> MRRRIPSRTPGSGAKQKSWFPRRSL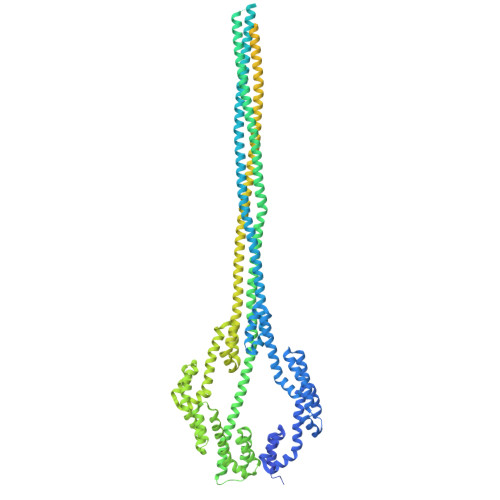QVLLSAGMLSGLLGTPAALAAEPAPLPANVRADIVGYWETGGAGLKAAAEQALLGGDEAIRKFLADAPSIQHDDNRIDAARMAMTGGSGLRQAAKDAIRLSPAELEKFLLYGYEEPLDDDHKVEIARLINLGGPGVREAGKAALQGTAEERELFLNSGQYTAQQDDNRVDVARLATTGGPNVQAAAKVALRGTPEDMVEFLEVGQFTARNRDQEHATIAELIKQAELAGKQADDARKTAEESSKKAVDASQLAKEAAQKAAEETEAAKDDSQKAAVKAKQAADAARAAADAAQEAIGSANAANRAARRAALAAAQTASAATAAAEAANKAYKAAIAAAGDEGKADEAKEAAKQARAAADAATKSGLAAENAGLASAAAATASTAAKSASSNARAAAGAAEEANQHADAAGVHSNEAALAAAEARRHADAADRAADRSSALAQRAATAAYGARDAANSAAEHANKAADYADESAAHAGDSAAYAATAKRNAQAAQEAAKTATAAVTKANEIFKLARETETANLETRTDAAIERARSMKSASETSITASATTQVEALALNDTATELAKEASRPDIDVQATAAKGRQLAMQAMKLLGPWHQEAAARALSGTDQDVLDYLRTRWKEANHNDIRQQIVDLSTQSPYASVRTAAAEALNGTPEQIEAFHTTGQYTAGSDDMKVDVARLANTGGPGVSQAAKTALADGTGKTLATFLQIGQYGERLSDEKVVTARLAETGSPEVQAAAKIALAGPPELLHEFVTTGQYMAKRKDDLADVHVNQVERLLAEGSLIAAEANEDAWRATEAAATAEGAAADAATAAEKAEASAAQAKQHAADADASADAATRSAADAAASAATARDAADRAAQDATAAENSAAEAAFSAAYARDSASKADDAADRARASALAAGKSADEAEAEAKEAWKTTRALAEKEAEEARRKAAEERKRQQEQAGEPKRVCIPHPTRETMIPIMPCAASPDDSMIMPGPVDPTIRAVVWELAGLNDIKACIDKPLSGNCVMAVVGVTPWGKFKLVSKLGNGLDAVKDARGARRTVACLTGAAHSFPAGTRVLMADGTRRSIEQIEAGDLVTATDPTTGETGARTVTRTIHTPDDRNFTDVALADGSTLTSTTHHPYWSQNDQTWKNAGDLEAGDTLRTPQNTAVVIAATHDWPGLQDAYDLTVDGFHSYYVSTGTTDVLVHNNDNPCPDWVSKAWKKLPKRKSGDPTSGYVFEADGTLVWDSVLTSGRSPLSEDISAFLKGSPDFPNFPGYADVAHHAEAKIAWEMRTKMGKGKKLHIVINTNYVCPKVSSPNSMGCKQAVPAILYEDQTLYVHYPGASDALELKGTAKR> MHHHHHHETSEERAARLAKMSAYAAQRLANESPEQRATRLKRMSEYAAKRLSSETREQ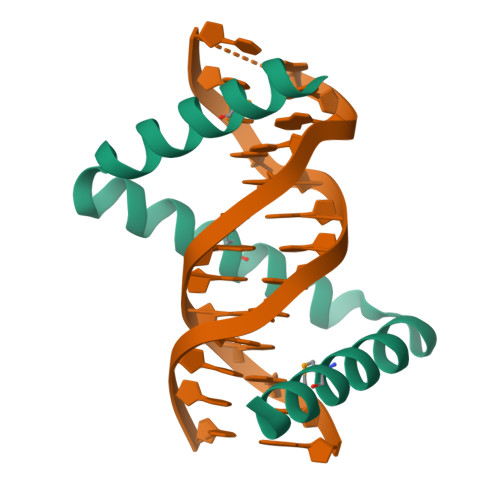RAIRLARMSAYAARRLANETPAQRQARLLRMSAYAAKRQASKKS>[2x]TISVRVTTMDAELEFAIQPNTTGKQLFDQVVKTIGLREVWFFGLQYQDTKGFSTWLKLNKKVTAQDVRKESPLLFKFRAKFYPEDVSEELIQDITQRLFFLQVKEGILNDDIYCPPETAVLLASYAVQSKYGDFNKEVHKSGYLAGDKLLPQRVLEQHKLNKDQWEERIQVWHEEHRGMLREDAVLEYLKIAQDLEMYGVNYFS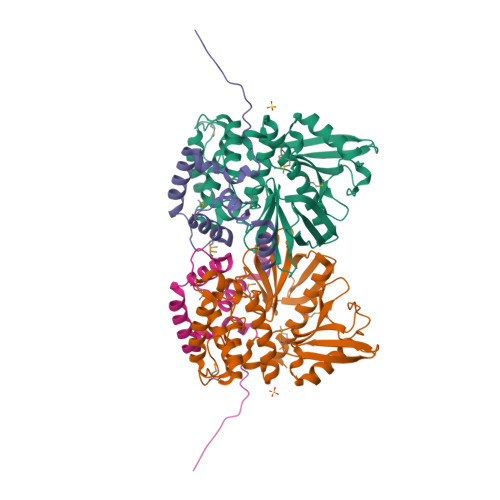IKNKKGSELWLGVDALGLNIYEQNDRLTPKIGFPWSEIRNISFNDKKFVIKPIDKKAPDFVFYAPRLRINKRILALCMGNHELYMRRRKP;>AEASADLRADAMAKDRSEEERTTEAEKNERVQKHLKALTSELANARDESKKTANDMIHAENMRLGRDKYKTLRQIRQGNTKQRIDEFESM[2x]>ATMGDEFVCEENEPFTCNQTKLFNSGNFEKGFIFGVASSAYQVEGGRGRGLNVWDSFTHRFPEKGGADLGNGDTTCDS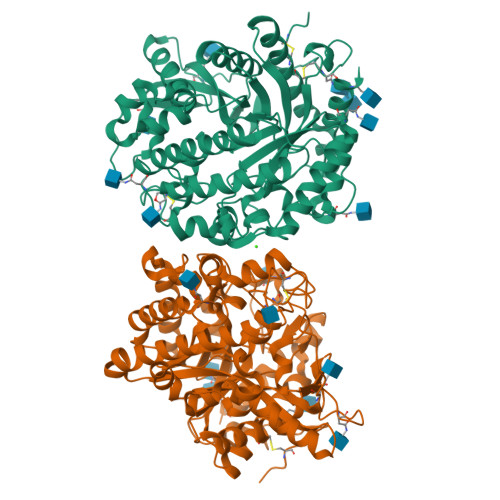YTLWQKDIDVMDELNSTGYRFSIAWSRLLPKGKRSRGVNPGAIKYYNGLIDGLVAKNMTPFVTLFHWDLPQTLQDEYNGFLNKTIVDDFKDYADLCFELFGDRVKNWITINQLYTVPTRGYALGTDAPGRCSPKIDVRCPGGNSSTEPYIVAHNQLLAHAAAVDVYRTKYKDDQKGMIGPVMITRWFLPFDHSQESKDATERAKIFFHGWFMGPLTEGKYPDIMREYVGDRLPEFSETEAALVKGSYDFLGLNYYVTQYAQNNQTIVPSDVHTALMDSRTTLTSKNATGHAPGPPFNAASYYYPKGIYYVMDYFKTTYGDPLIYVTENGFSTPGDEDFEKATADYKRIDYLCSHLCFLSKVIKEKNVNVKGYFAWSLGDNYEFCNGFTVRFGLSYVDFANITGDRDLKASGKWFQKFINVTDEDSTNQDLLRSSVSSKNRDRKSLADALEGSENLYFQ[4x]> CPRFLKVKNWETDVVLTDTLHLKSTLETGCTE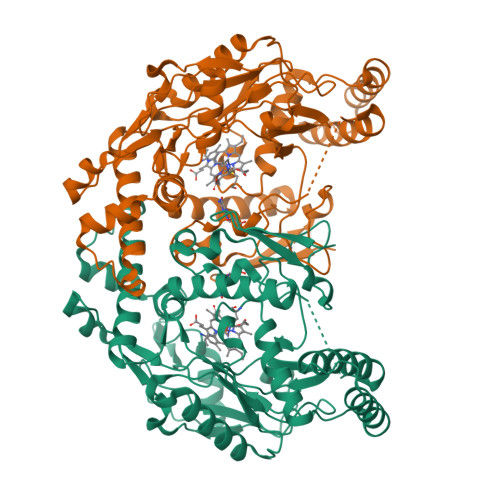HICMGSIMLPSQHTRKPEDVATKDQLFPLAKEFLDQYYSSIKRFGSKAHMDRLEEVNKEIESTSTYQLKDTELIYGAKHAWRNASRCVGRIQWSKLQVFDARDCTTAHGMFNYICNHVKYATNKGNLRSAITIFPQRTDGKHDFRVWNSQLIRYAGYKQPDGSTLGDPANVQFTEICIQQGWKAPRGRFDVLPLLLQANGNDPELFQIPPELVLEVPIRHPKFDWFKDLGLKWYGLPAVSNMLLEIGGLEFSACPFSGWYMGTEIGVRDYCDNSRYNILEEVAKKMDLDMRKTSSLWKDQALVEINIAVLYSFQSDKVTIVDHHSATESFIKHMENEYRCRGGCPADWVWIVPPMSGSITPVFHQEMLNYRLTPSFEYQPDPWNTHVWKG> MHHHHHHSSGRENLYFQGMSEVIVPRSFRLLDELERGQKGNVSEGVSFGLESADDITLSNWSCTIFGQPGTVFENRIYSLTIFCDDNYPDSPPTVKFDTKIEMSCVDNCGRVIKNNLHILKNWNRNYT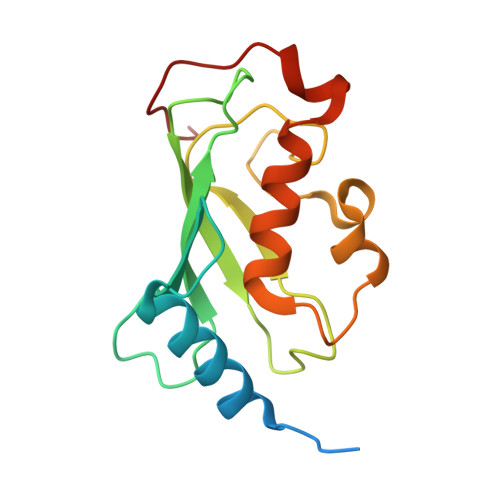IETILISLRQEMLSSANKRLPQPNEGEVYS(S)-{1-[(2,5-dimethylphenyl)methyl]-1H-benzimidazol-2-yl}(pyridin-4-yl)methanol | C22 H21 N3 O | 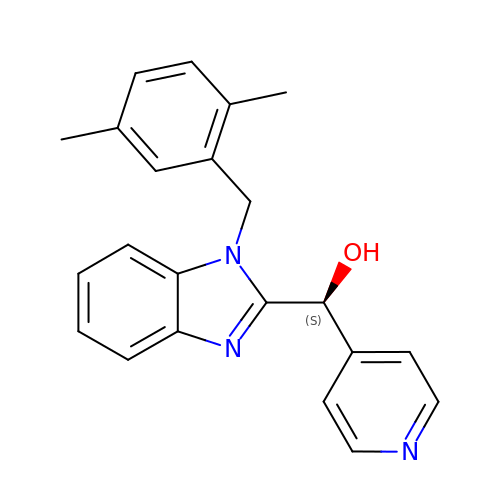MKABLXAUPLCAHG-NRFANRHFSA-N>[2x]ANHHHHHHPCCSNPCQNRGECMSTGFDQYKCDCTRTGFYGENCTTPEFLTRIKLLLKPTPNTVHYILTHFKGVWNIVNNIPFLRSLIMKYVLTSRSYLIDSPPTYNVHYGYKSWEAFSNLSYYTRALPPVADDCPTPMGVKGNKELPDSKEVLEKVLLRREFIPDPQGSNMMFAFFAQHFTHQFFKTDHKRGPGFTRGLGHGVDLNHIYGETLDRQHKLRLFKDGKLKYQVIGGEVYPPTVKDTQVEMIYPPHIPENLQFAVGQEVFGLVPGLMMYATIWLREHNRVCDILKQEHPEWGDEQLFQTSRLILIGETIKIVIEDYVQHLSGYHF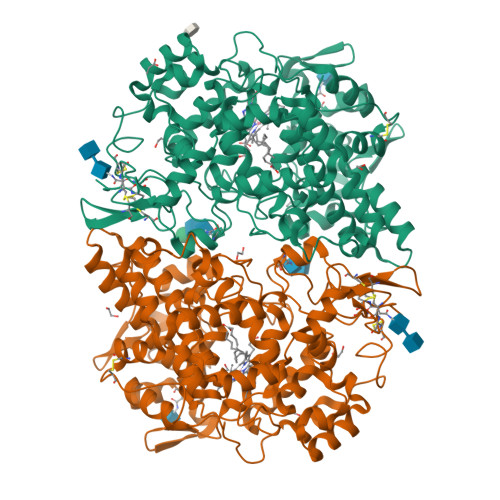KLKFDPELLFNQQFQYQNRIASEFNTLYHWHPLLPDTFNIEDQEYSFKQFLYNNSILLEHGLTQFVESFTRQIAGRVAGGRNVPIAVQAVAKASIDQSREMKYQSLNEYRKRFSLKPYTSFEELTGEKEMAAELKALYSDIDVMELYPALLVEKPRPDAIFGETMVELGAPFSLKVLMGNPICSPQYWKPSTFGGEVGFKIINTASIQSLICNNVKGCPFTSFNVQDPQPTKTATIAASASHSRLDDINPTVLIKRRSTEL>[2x]GSSGSSGMSLLTEVETYVLSIIPSGPLKAEIAQKLEDVFAGK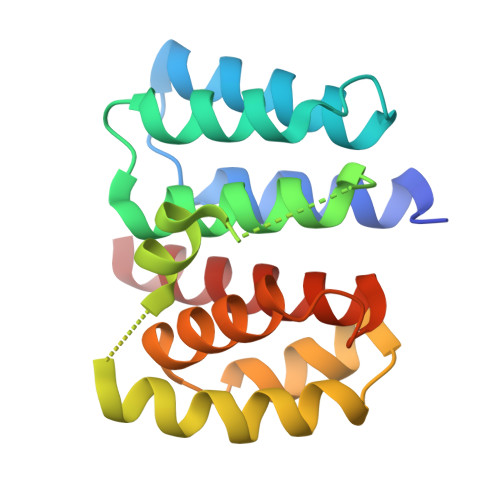NTDLEALMEWLKTRPILSPLTKGILGFVFTLTVPSERGLQRRRFVQNALNGNGDPNNMDRAVKLYKKLKREITFHGAKEVALSYSTGALASCMGLIYNRMGTVTTEVAFGLVCATCEQIADSQ>MGSHHHHHHGARQMATPASAPDTRALVADFVGYKLRQKGYVSGAGPGEGPAADPLHQAMRAAGDEFETRFRRTFSDLAAQLHVTPGSAQQRFTQVSDELFQGGPNWGRLVAFFVFGAALCAESVNKEMEPL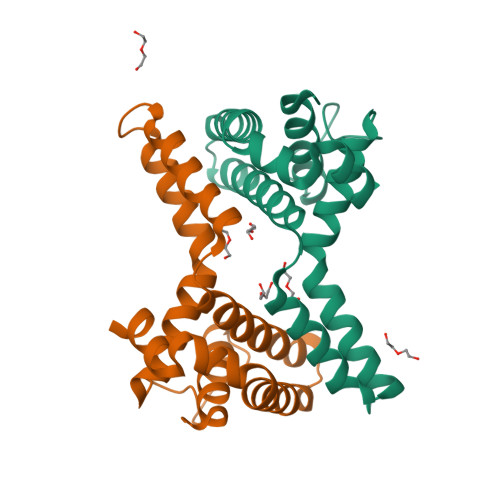VGQVQEWMVEYLETRLADWIHSSGGWAEFTALYGDGALEEARRLRE[2x]> HGREFVNDIWSRLKTDEDRAVVKKMVEQTGHIDKFKKFGQLDFIDNNIVVKTDDEKEIFDQIVVRDMTLKTLEDDLQEVQEISLPLFKKKLELLEVYLGWLDNVYTEMRKLDDDAASHVECGKEDSKGTKRKKKKNSSRSRARKNICGYCSTYERIPCS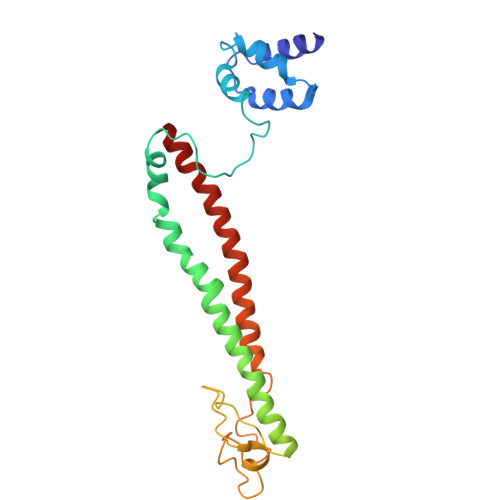VEEFVRDFGSNEEATKIHEVCTKWKCNRHLDWVSTNQEQYLQQIDSLESMQERLQHLIQARKKQLNIQYYEEILRRGL> GGEYEWEYDEEEEKNQLEIERLEEQLSINVYDYNCHVDLIRLLRLEGELTKVRMARQKMSEIFPLTEELWLEWLHDEISMAQDGLDREHVYDLFEKAVKDYICPNIWLEYGQYSVGGIGQKGGLEKVRSVFERALSSVGLHMTKGLALWEAYREFESAIVEAARLEKVHSLFRRQLAIPLYDMEATFAEYEEWSEDPIPESVIQNYN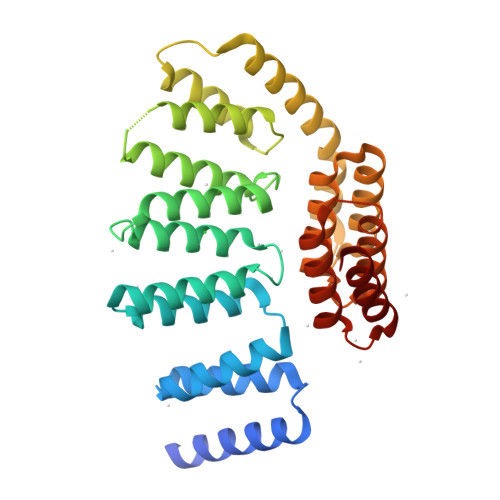KALQQLEKYKPYEEALLQAEAPRLAEYQAYIDFEMKIGDPARIQLIFERALVENCLVPDLWIRYSQYLDRQLKVKDLVLSVHNRAIRNCPWTVALWSRYLLAMERHG> MNIQTTVEPTSAERAEKLQGMGCKRKRVEDIRFTQGKGNYVDDVKLPGMLFGDFVRSS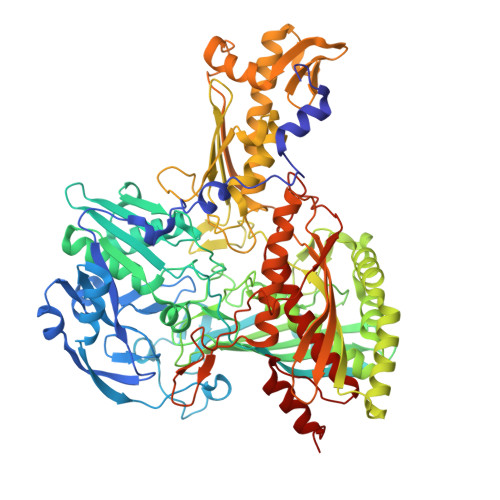HAHARIKSIDTSKAKALPGVFAVLTAADLKPLNLHYMPTLAGDVQAVLADEKVLFQNQEVAFVVAKDRYVAADAIELVEVDYEPLPVLVDPFKAMEPDAPLLREDIKDKMTGAHGARKHHNHIFRWEIGDKEGTDATFAKAEVVSKDMFTYHRVHPSPLETCQCVASMDKIKGELTLWGTFQAPHVIRTVVSLISGLPEHKIHVIAPDIGGGFGNKVGAYSGYVCAVVASIVLGVPVKWVEDRMENLSTTSFARDYHMTTELAATKDGKILAMRCHVLADHGAFDACADPSKWPAGFMNICTGSYDMPVAHLAVDGVYTNKASGGVAYRCSFRVTEAVYAIERAIETLAQRLEMDSADLRIKNFIQPEQFPYMAPLGWEYDSGNYPLAMKKAMDTVGYHQLRAEQKAKQEAFKRGETREIMGIGISFFTEIVGAGPSKNCDILGVSMFDSAEIRIHPTGSVIARMGTKSQGQGHETTYAQIIATELGIPADDIMIEEGNTDTAPYGLGTYGSRSTPTAGAATAVAARKIKAKAQMIAAHMLEVHEGDLEWDVDRFRVKGLPEKFKTMKELAWASYNSPPPNLEPGLEAVNYYDPPNMTYPFGAYFCIMDIDVDTGVAKTRRFYALDDCGTRINPMIIEGQVHGGLTEAFAVAMGQEIRYDEQGNVLGASFMDFFLPTAVETPKWETDYTVTPSPHHPIGAKGVGESPHVGGVPCFSNAVNDAYAFLNAGHIQMPHDAWRLWKVGEQLGLHV>MPVVKINAIEVPAGAGPELEKRFAHRAHAVENSPGFLGFQLLRPVKGEERYFVV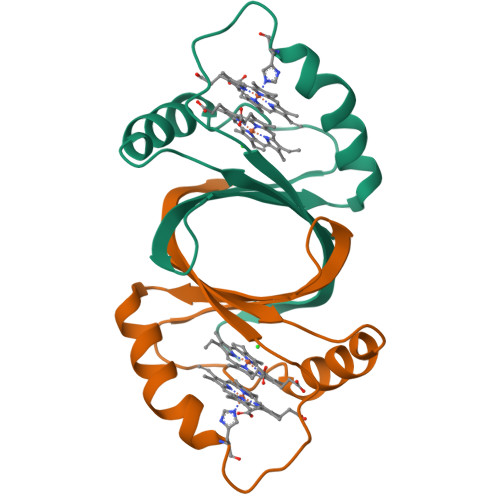THWESDEAFQAWANGPAIAAHAGHRANPVATGASLLEFEVVLDVGGTGKTAGGVPRGKLAAALEHHHHHH[2x]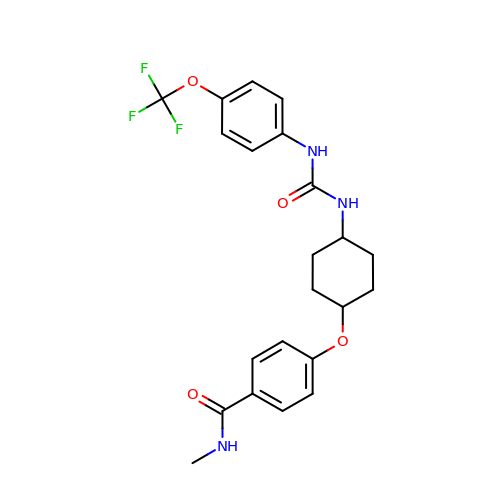N-methyl-4-{[trans-4-({[4-(trifluoromethoxy)phenyl]carbamoyl}amino)cyclohexyl]oxy}benzamide | C22 H24 F3 N3 O4 | JNPWHXLRBKEIPP-RZDIXWSQSA-N>QAKHKQRKRLKSSCKRHPLYVDFSDVGWNDWIVAPPGYHAFYCHGECPFPLADHLNSTNHAIVQTLVNSVNSKIPKACCVPTELSAISMLYLDENEKVVLKNYQDMVVEGCGCR[2x];> ETGSPCKILKCNSEFWSATSGSHAPASDDTPEFCAALRSYA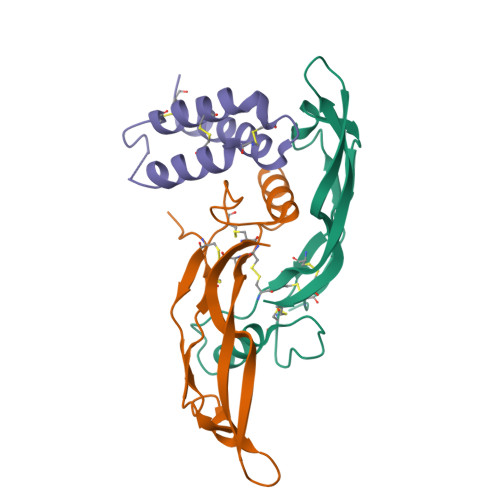LCTRRTARTCRGDLAYHSAVHGIEDLMSQHNCSKDGPTSQPRLRTLPPAGDSQERSGTKHHHHHH Rspo (R-spondin, also roof plate-specific spondin) proteins are evolutionarily conserved from fish to humans and have well-documented roles in a broad range of developmental and physiological processes resulting from enhancement of canonical and non-canonical Wnt signalling. ZNRF3/RNF43 specifically targets these Wnt receptors for ubiquitination and turnover, hence reducing Wnt signalling responses. Direct extracellular interaction with Rspo proteins inhibits ZNRF3/RNF43 activity. Here we report a molecular level analysis of the ZNRF3/RNF43 ectodomain structure and its interactions with Rspo proteins.

By using a combination of heavy atom and molecular-replacement-based phasing strategies, we determined multiple crystal structures for Xenopus (x) Rspo2Fu1–Fu2 (highest resolution 2.2 Å), xZNRF3ecto, zebrafish (z) ZNRF3ecto and mouse (m) ZNRF3ecto, (highest resolutions 2.4, 1.6 and 2.0 Å, respectively), plus complexes comprising xZNRF3ecto–xRspo2Fu1–Fu2, mZNRF3ecto–mRspo2Fu1–Fu2, mZNRF3ecto–xRspo2Fu1–Fu2 and xRNF4F3ecto–xRspo2Fu1–Fu2 (at 2.1, 2.8, 2.4 and 2.7 Å, respectively). The ZNRF3ecto crystal structures revealed a distinctive variant of the protease-associated domain topology. Two β-sheets (comprising β2, β1, β7, β3 and β4, β5, β6 strands, respectively) splay apart, accommodating an α-helix (αC) at the open edge; two additional α-helices (αA and αB) pack against the β4, β5 and β6 face of this distorted β-sandwich. A disulphide bridge, conserved across species, links two structurally elaborate loops, β3–β4 and β4–αA. The crystal structures for apo xZNRF3ecto, zZNRF3ecto and mZNRF3ecto showed no major differences in the main chain conformation. Comparisons of ZNRF3ecto structures for proteins crystallized in several different crystal lattices, or for crystals containing multiple copies in the asymmetric unit, consistently highlighted an acidic region (N105-E114; residue numbering is for mouse sequences unless otherwise stated) within the β3–β4 loop, the short αC–β7 loop and the extended β1–β2 hairpin as flexible elements of the fold. All but two of these crystal structures reveal an extensive interface (average interface area 992±109 Å2) formed between two ZNRF3ecto polypeptide chains. The interaction is twofold symmetric; strands β3 and β7 of the ‘subunits’ abut face-to-face at the core of the dimer. The β1–β2 hairpin forms a second interface by reaching out to embrace helix αA and the β3–β4 loop in the opposing subunit. Intriguingly, these structural features interact in a parallel (cis) fashion consistent with ZNRF3 associating as a dimer on the cell surface.

>[2x]ETGKETAFVEVVLFESSPSGDYTTHTTGLTGRFSRAGAMLSAEGEIVQMHPLGLCNNNDEEDLYEYGWVGVVKLEQPELDPKPCLTVLGKAKRAVQRGATAVIFDVSENPEAIDQLNQGSEDPLKRPVVYVKGADAIKLMNIVNKQKVARARIQHLGTKHHHHHH>[4x]LHRNSLIVLADVALFLALYHFLPFEHNVVLGISMLAFIAVLWLTEALHVTVTAILVPVMAVFFGIFETQAALNNFANSIIFLFLGGFALAAAMHHQGLDKVIADKVLAMAQGKMSVAVFMLFGVTALLSMWISNTATAAMMLPLVLGVLSKVDADKQRST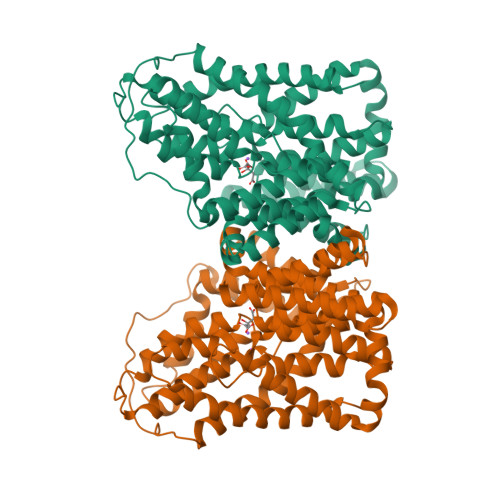YVFVLLGVAYSASIGGIATLVGSPPNAIAAAEVGLSFTDWMKFGLPTAMMMLPMAIAILYFLLKPTLNGMFELDRAPVNWDKGKVVTLGIFGLTVFLWIFSSPINAALGGFKSFDTLVALGAILMLSFARVVHWKEIQKTADWGVLLLFGGGLCLSNVLKQTGTSVFLANALSDMVSHMGIFVVILVVATFVVFLTEFASNTASAALLIPVFATVAEAFGMSPVLLSVLIAVAASCAFMLPVATPPNAIVFASGHIKQSEMMRVGLYLNIACIGLLTAIAMLFWQ>MAEAAAAAAAAAAAGETSASSGSAAERDPDQDRAGRRLRVLSGHLLGRPQEALSTNECKARRAASAATAAPTATPAAPESGIIPKKRQELMKWNGWGYNDSKFFLNKKGQLELTGKRYPLSGVALPTFKDWIQNTFGINLDHKTTSKASLNPSDTPPSIVNEDFLHELKKTNISYSQEADDRVFRAHGHCLHEIFLLREGMFERIPDIVLWPTCHDDVVKIVNLACKYNLCIIPIGGGTSVSYGLMCPADETRTIISLDTSQMNRILWVDENNLTAHVEAGITGQELERQLKESGYCTGHEPDSLEFSTVGGWISTRASGMKKNIYGNIEDLVVHMKVVTPRGVIEKSCQGPRMSTGPDIHHFIMGSEGTLGVITEATIKIRPTPEYQKYGSVAFPNFEQGVACLREIAKQRCAPASIHLMDNQQFQFGHALKPQVSSIFTSFLDGLKKFYITKFKGFDPNQLSVATLLFEGDREKVLQHEKQVYDIAAKFGGLAAGEDNGQRGYLLTYVIAYMRDLGLEYYIIGESFETS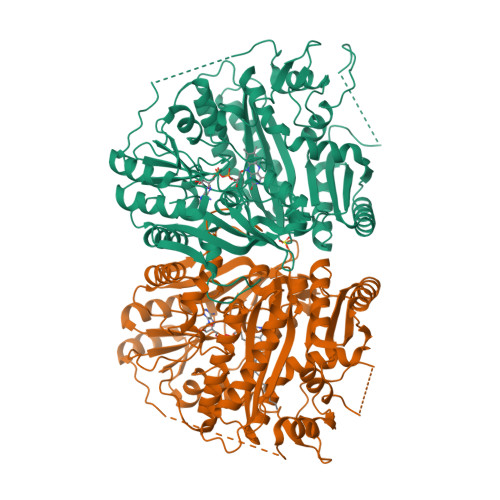APWDRVVDLCRNVKERIRRECKEKGVQFPPLSTCRVTQTYDAGACIYFYFAFNYRGISDPLAVFEQTEAAAREEILANGGSLSHHHGVGKLRKQWLKESISDVGFGMLKSVKDYVDPTNIFGNRNLL[4x]>GPLGSPEFDCHLSDMLQQLHSVNASKPSERGLVRQEEAEDPACIPIFWVSKWVDYSDKYGLGYQLCDNSVGVLFNDSTRLILYNDGDSLQYIERDGTESYLTVSSHPNSLMKKITLLKYFRNYMSEHLLKAGANITPREGDELARLPYLRTWFRTRSAIILHLSNGSVQINFFQDHTKLILC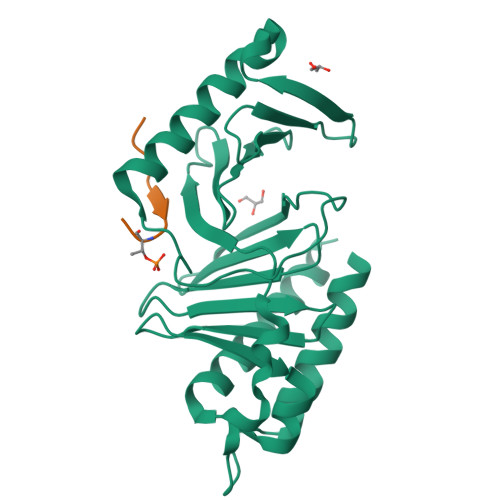PLMAAVTYIDEKRDFRTYRLSLLEEYGCCKELASRLRYARTMVDKLLSSR[3x];>XFDPPLHSTAX[3x]>MNHKAFAKFPSSASISPNPFTVSIPDEQLDDLKTLVRLSKIAPPTYESLQADGRFGITSEWLTTMREKWLSEFDWRPFEARLNSFPQFTTEIEGLTIHFAALFSEREDAVPIALLHGWPGSFVEFYPILQLFREEYTPETLPFHLVVPSLPGYTFSSGPPLDKDFGLMDNARVVDQLMKDLGFGSGYIIQGGDIGSFVGRLLGVGFDACKAVHLNFCNMSAPPEGPSIESLSAAEKEGIARMEKFMTDGYAYAMEHSTRPSTIGHVLSSSPIALLAWIGEKYLQWVDKPLPSETILEMVSLYWLTESFPRAIHTYREWVPTASAPNGATPYQKELYIHKPFGFSFFPKDLVPVPRSWIATTGNLVFFRDHAEGGHFAAL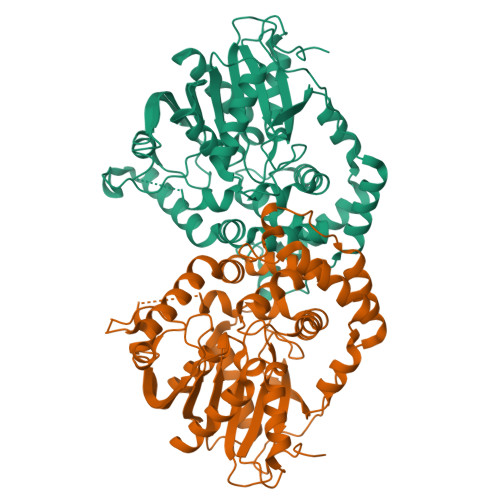ERPRELKTDLTAFVEQVWQKGRSHHHHHH[2x]>SNAQSNPNQELGVVQCLCRRIAPLTQPPFGVRCRATLNCPCDYIGDCPGPAEQYMYRCPNCGPRSHVACSGVHQGTCQQVHP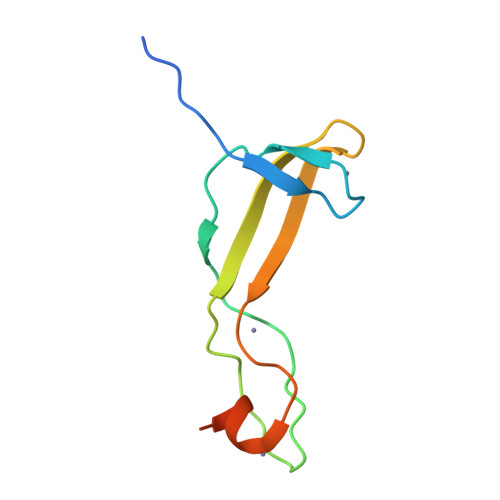GKDSVEYGG[2x]>MKRVITLFAVLLMGWSVNAWSFACKTANGTAIPIGGGSANVYVNLAPVVNVGQNLVVDLSTQIFCHNDYPETITDYVTLQRGSAYGGVLSNFSGTVKYSGSSYPFPTTSETPRVVYNSRTDKPWPVALYLTPVSSAGGVAIKAGSLIAVLILRQTNNYNSDDFQFVWNIYANNDVVVPTGGCDVSARDVTVTLPDYP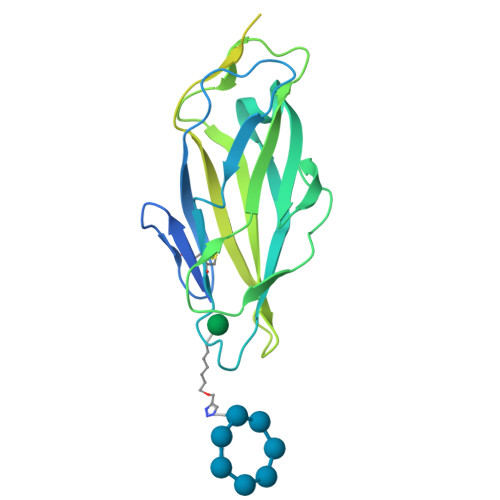GSVPIPLTVYCAKSQNLGYYLSGTTADAGNSIFTNTASFSPAQGVGVQLTRNGTIIPANNTVSLGAVGTSAVSLGLTANYARTGGQVTAGNVQSIIGVTFVYQ[2x]2-[(3-tert-butyl-1-phenyl-1H-pyrazol-5-yl)amino]-2-oxoethyl 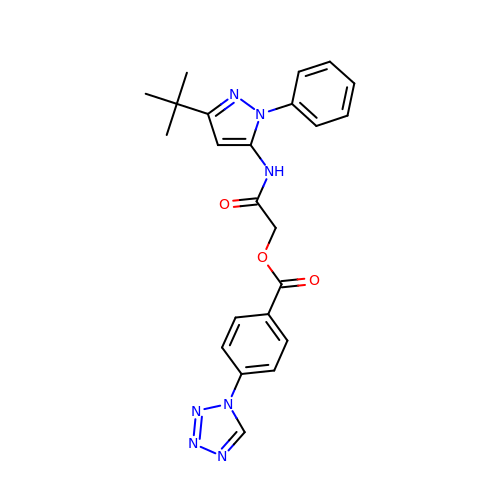4-(1H-tetrazol-1-yl)benzoate | C23 H23 N7 O3 | PRZQRZSCFWKYBL-UHFFFAOYSA-N>MFKDGSLIPYLTAGDPDKQSTLNFLLALDEYAGAIELGIPFSDPIADGKTIQESHYRALKNGFKLREAFWIVKAFRRHSSTPIVLMTYYNPIYRAGVRNFLAEAKASGVDGILVVDLPVFHAKEFTEIAREEGIKTVFLAAPNTPDERLKVIDDMTTGFVYLVSLYGTTGAREEIPKTAYDLLRRAKRICRNKVAVGFGVSKREHVVSLLKEGANGVVVGSALV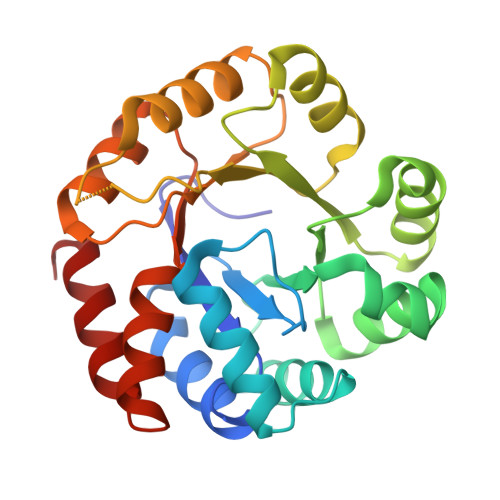KIIGEKGREATEFLKKKVEELLGI[2x]> MD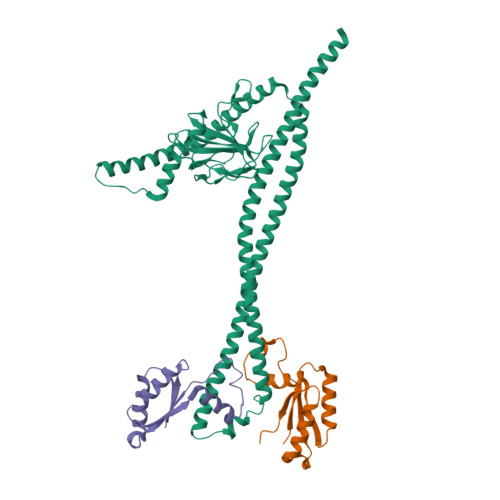ERDQLKSIQADIAAKERAVRQKQQQRASLLAQLKKQEEAISEATRKLRETQNTLNQLNKQIDEMNASIAKLEQQKAAQERSLAAQLDAAFRQGEHTGIQLILSGEESQRGQRLQAYFGYLNQARQETIAQLKQTREEVAMQRAELEEKQSEQQTLLYEQRAQQAKLTQALNERKKTLAGLESSIQQGQQQLSELRANESRLRNSIARAEAAAKARAEREAREAQAVRDRQKEATRKGTTYKPTESEKSLMSRTGGLGAPRGQAFWPVRGPTLHRYGEQLQGELRWKGMVIGASEGTEVKAIADGRVILADWLQGYGLVVVVEHGKGDMSLYGYNQSALVSVGSQVRAGQPIALVGSSGGQGRPSLYFEIRRQGQAVNPQPWLGR;>[2x]MGQITVYLQKTLDDDAAAGVVAQLQAEQGVEKVNYLSREDALGEFRNWSGFGGALDMLEENPLPAVAVVIPKLDFQGTESLNTLRDRITQINGIDEVRMDDSLEHHHHHH>[4x]GPHMRYVEIHRNL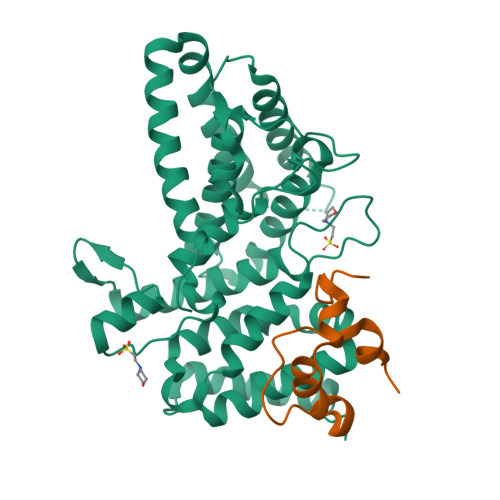KGLRKYMAEQAKTNLKLKQRMGDMRREIRKSVGQLTTGGMAANKDKQQKIKSILTEALSNQVESALVDPNNFVVEPRKPVEGATNNDPLLPSIFVYLINIFAKAAISQFINEAGARPETADPVGICVAAILSEPDFLWRGASLIDILIAKFRIVCPVLFGYRGSEKTEQGRQRLGWWKESGQWISEQQHMDRMTGLGAGFAAISLRKFALSKKQNPYPPRFYWMAMAKIVNTPPAEISNTQCVVLKAMVQNYEAKFIEFYGSAAIAALRTALIDFPARAPHKSAAVNSLEVLAQMLKRDTGLDLG;>[4x]GPHMGSPEFDGTLVRIWMPDGAPAYTADTEAEDPKVYEDEGVKRQWQSFLEKGRFEGGMPEVPPRREWCVWDF> MDVQEQFEGYLREEVDLLNKFEDSHFKQLEIFYTKSQTDHVINKDKLQFNALPFHTTLYKEINGKRVRLGTLLNWTKAERLDTIRHESMIKDERLRRLIDFDYGWIDYAVVLQRYLDEGNTIESANILQFDGDFVNNIKHPTQKNNFLDIKVIKECETYILMKDDNGIRDPDILRAWELNSIPEVIELDVDGETKKFNLRKEMIKRIQDEAPVYFFCNPYRYAVANLDPNIPEVRLWLEYFIGSEDFFGFNGPNVIVSKSLLAAKRFEVVVNHLRKVAAFELDVESKEVMNEWIKYIMIDPVYRSYKNRGAFGNLNQHVFARTKSEGLSWSLIDIGTTNFELKPTKKVAGSYVNKFNLVDDVLVEESLKDLRNEGLHKMADVTRRMIDADITPENVKKGKLNRLALSYCGYTGSHSATAMVKQFNGTKDLDPNCDPMFVDIVKDNMRVYMQEGLQKYPQGSRKSNRLDILFKGGTSSASSTNEHAVVNGRFRYRSELYRERDVNSSTVFKTATPGQYRVVKKISAKLKSKNANIVTHPMNFINFKVDDLDIVVNAGSRLVRGTRAKRIITPNYGTIYAASLMTVLPAVRLLSSRASNMGALSTQGRIGTTYHGALPHDVMAPQLAVTSSDDVSKICVAKDFGQFDTSQWGQISKAHADGVRSMKAHYSMGHDTLVDLDLNDASFADLLEVTAMSYERPLKYKMNGLVCESAGVKSGELTTQTRNTTTNISHSTVALDDYNNRAYRLNLPKLELVTDNKVGDDSVEVLRVVDGSPLTPEIAKLYVNCMQDHADKNHLEISAKRTIVGNNVAEHIKIWVFKGYLALDVFLDSVTSEKNSFSNLNYLEQVNILYDMAMTLMIRYCSVQACMTQFCNDMKLLNGIRAGNYTFIPTPKIICAYGTPEICLRAPE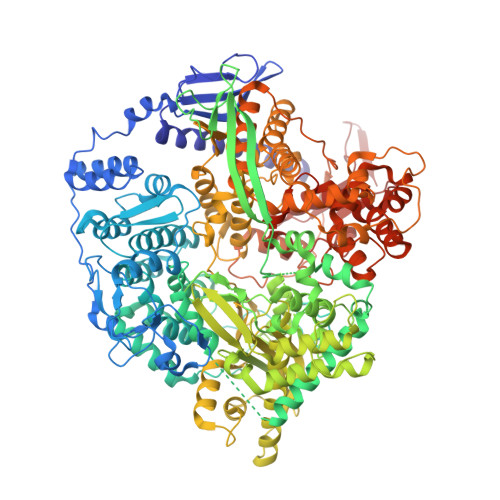IRSFGRYLPIDEDEYSVLNDLVASLSTNKPKMDFVAQMFEQNGNQVHGIWLDHFKRKNDVNPDGGGIHISEGLKRLMPEYCERHLNELVYKTLDDKVIRDYTSDIIITNICKGKLSKAPKLAFFANFYLSLTGFNGVDSPYLTADEGVKNVHRVIGLSYRNTLSTSPTANVDRILRNNPGSAPAYLTGNDILGVLSDYPYQNWRTVVELLDITEPSATAIIEVATNQMHAYLADKDLNTANLFDNTSRTYDISDRTYPKFVNITSNLSNSNRRGFQLEAMKHIIYMARRGIATLANTHPSKIGNTVYYDY> VKDTYTDRLDDWNGIIAGNQYYDSKNDQMAKLNQELEGKVADSLSSISSQADRIYLWEKFSNYKTSANLTATYRKLEEMAKQVTNPSSRYYQDETVVRTVRDSMEWMHKHVYNSEKSIVGNAADYEIGTPRAINNTLSLMKEYFSDEEIKKYTDVIEKFVPDPEHFRKTTDNPFKALGGNLVDMGRVKVIAGLLRKDDQEISSTIRSIEQVFKLVDQGEGFYQDGSYIDHTNVAYTGAYGNVLIDGLSQLLPVIQKTKNPIDKDKMQTMYHWIDKSFAPLLVNGELMDMSRGRSISRANSEGHVAAVEVLRGIHRIADMSEGETKQRLQSLVKTIVQSDSYYDVFKNLKTYKDISLMQSLLSDAGVASVPRTSYLSAFNKMDKTAMYNAEKGFGFGLSLFSSRTLNYEHMNKENKRGWYTSDGMFYLYNGDLSHYSDGYWPTVNPYKMPGTTETDAKRADSDTGKVLPSAFVGTSKLDDANATATMDFTNWNQTLTAHKSWFMLKDKIAFLGSNIQNTSTDTAATTIDQRKLESSNPYKVYVNDKEASLTEQEKDYPETQSVFLESSDSKKNIGYFFFKKSSISMSKALQKGAWKDINEGQSDKEVENEFLTISQAHKQNGDSYGYMLIPNVDRATFNQMIKELESSLIENNETLQSVYDAKQGVWGIVKYDDSVSTISNQFQVLKRGVYTIRKEGDEYKIAYYNPETQESAPDQEVFKK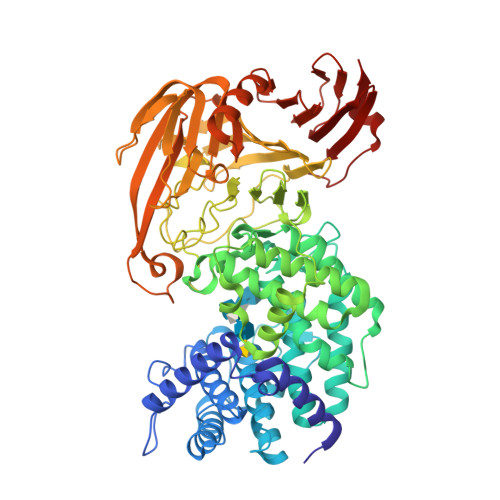L4-[3-cyano-6-(3-methoxyphenyl)-2-oxo-1H-pyridin-4-yl]benzoic acid | C20 H14 N2 O4 | 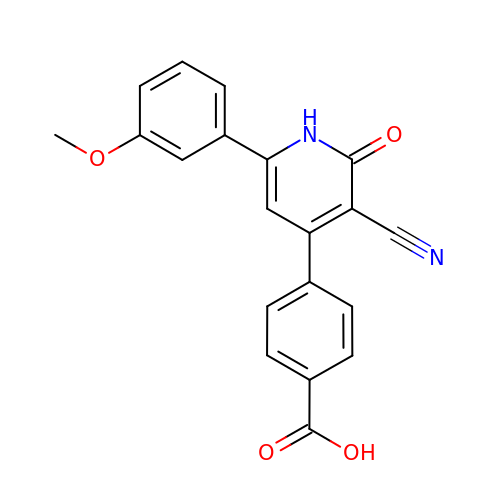DYVOFZNYRIDQOP-UHFFFAOYSA-N>[2x]SHVEYSRITKFFQEQPLEGYTLFSHRSAPNGFKVAIVLSELGFHYNTIFLDFNLGEHRAPEFVSVNPNARVPALIDHGMDNLSIWESGAILLHLVNKYYKETGNPLLWSDDLADQSQINAWLFFQTSGHAPMIGQALHFRYFHSQKIASAVERYTDEVRRVYGVVEMALAERREAL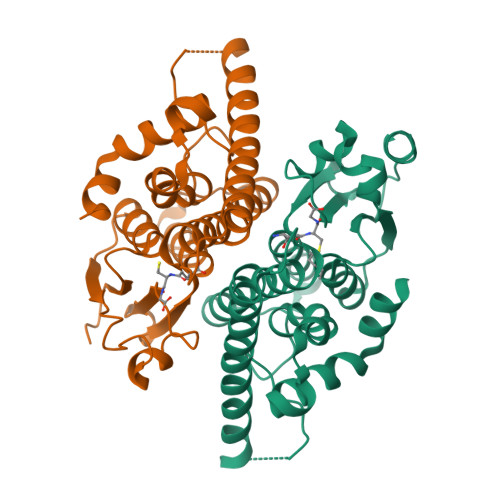VMELDTENAAAYSAGTTPMSQSRFFDYPVWLVGDKLTIADLAFVPWNNVVDRIGINIKIEFPEVYKWTKHMMRRPAVIKALRGE4-[(9-cyclopentyl-7,7-difluoro-5-methyl-6-oxo-6,7,8,9-tetrahydro-5H-pyrimido[4,5-b][1,4]diazepin-2-yl)amino]-2-fluoro-5-methoxy-N-(1-methylpiperidin-4-yl)benzamide | C27 H34 F3 N7 O3 | 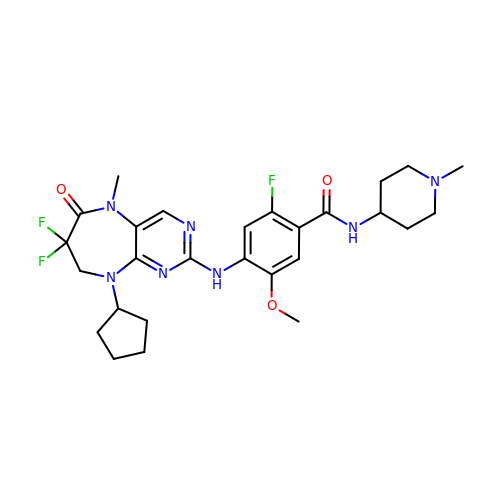GWRSATNRNFYMDI-UHFFFAOYSA-N> MDAV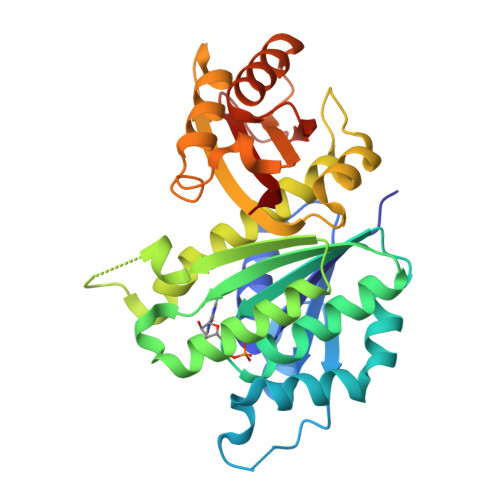IKVIGVGGGGGNAVEHMVRERIEGVEFFAVNTDAQALRKTAVGQTIQIGSGITKGLGAGANPEVGRNAADEDRDALRAALEGADMVFIAAGMGGGTGTGAAPVVAEVAKDLGILTVAVVTKPFNFEGKKRMAFAEQGITELSKHVDSLITIPNDKLLKVLGRGISELDAFGAANDVLKGAVQGIAELITRPGLMNVDFADVRTVMSEMGYAMMGSGVASGEDRAEEAAEMAISSPLLEDIDLSGARGVLVNITAGFDLRLDEFETVGNTIRAFASDNATVVIGTSLDPDMNDELRVTVVATGIG> NKGSIEGREPAVYFKEQFLDGDGWTSRWIESKHKSDFGKFVLSSGKFYGDEEKDKGLQTSQDARFYALSASFEPFSNKGQTLVVQFTVKHEQNIDCGGGYVKLFPNSLDQTDMHGDSEYNIMFGPDICGPGTKKVHVIFNYKGKNVLINKDIRCKDDEFTHLYTLIVRPDNTYEVKIDNSQVESGSLEDDWDFLPGSGDPSIYAYDNFGVLGLDLWQVKSGTIFDNFLITNDEAYAEEFGNETWGVTKAAEKQMKDKQDEEQRLK

shown to play a key role in the MHC class I assembly pathway. cellular processes with broad patho-physiological implications. GSG linker and the C-terminal residues 369–417 were deleted. The long C-terminal α3 helix is kinked at Thr346.

to two different crystal forms in our study. yielded similar structures, except for their N-terminal extension.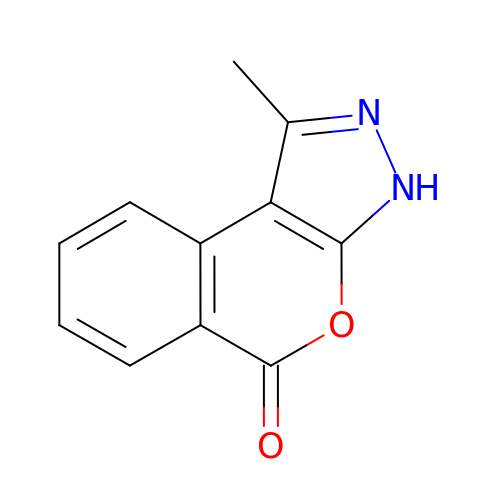1-methyl[2]benzopyrano[3,4-c]pyrazol-5(3H)-one | C11 H8 N2 O2 | UNIATRJVNFDJDH-UHFFFAOYSA-N> QDNSR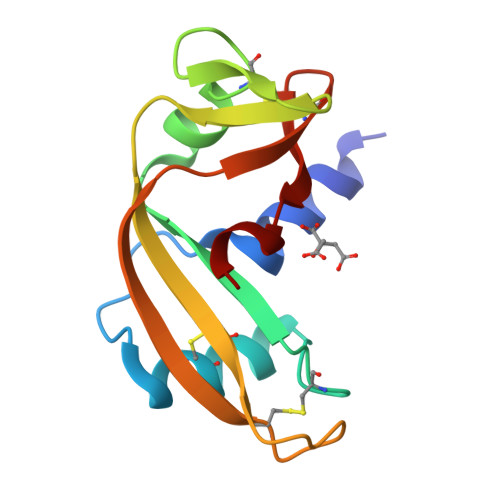YTHFLTQHYDAKPQGRDDRYCEAIMRRRGLAAPCKDINTFIHGNKRSIKAICENKNGNPHRENLRISKSSFQVTTCKLHGGAPWPPCQYRATAGFRNVVVACENGLPVHLDQSIFR> MPIEIKELHIKITVDDSNNAGRGGASSGEDKQQLVAQCVEQVLDVLKSQKE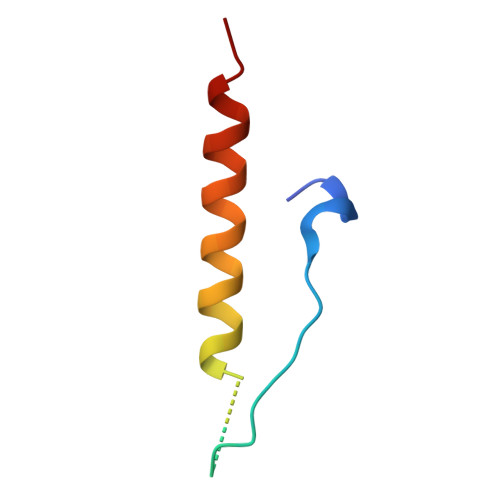R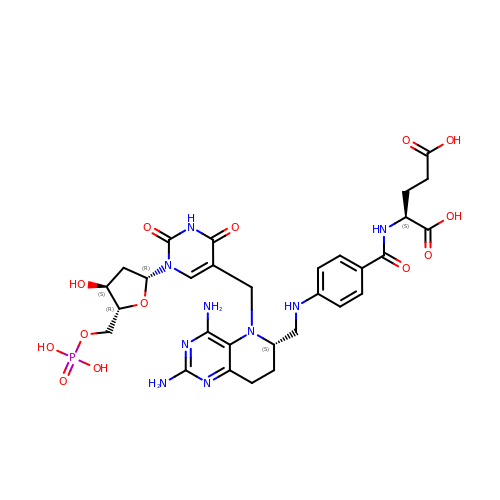(2S)-2-({4-[({(6S)-2,4-diamino-5-[(1-{(2R,4S,5R)-4-hydroxy-5-[(phosphonooxy)methyl]tetrahydrofuran-2-yl}-2,4-dioxo-1,2,3,4-tetrahydropyrimidin-5-yl)methyl]-5,6,7,8-tetrahydropyrido[3,2-d]pyrimidin-6-yl}methyl)amino]benzoyl}amino)pentanedioic acid (non-preferred name) | C30 H38 N9 O13 P | OYTZJQBUPHBEFY-GLOJMNGXSA-N>[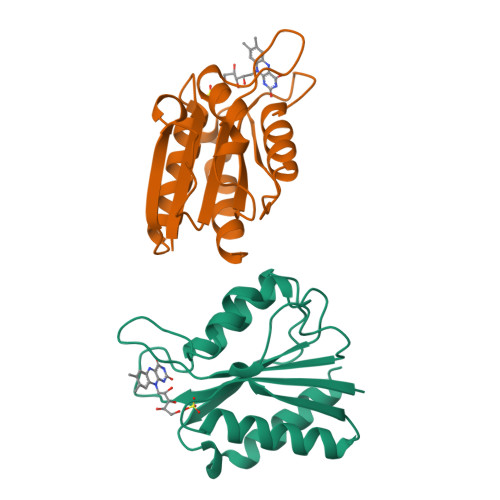2x]PKALIVYGSTTGNTEYTAETIARELADAGYEVDSRDAASVEAGGLFEGFDLVLLGCSTWGDDSIELQDDFIPLFDSLEETGAQGRKVACFGCGDSSYEYFCGAVDAIEEKLKNLGAEIVQDGLRIDGDPRAARDDIVGWAHDVRGAI After transcription, the 3′-end is oligo-uridylylated by a terminal uridylyltransferase, TUT1 (TUTase6)910, one of the members of the non-canonical nucleotidyltransferases. TUT1 is composed of N-terminal Zn-finger, RRM, palm, fingers and KA-1 domains. The C-terminal region of TUT1 is a previously unidentified RNA-binding domain, and it was named the KA-1 domain. Thus, the present structural and biochemical studies have demonstrated that TUT1 acts as a U6 snRNA-specific terminal uridylyltransferase.

The crystal of TUT1 lacking the N-terminal Zn-finger, PRR and C-terminal region (TUT1_ΔC) was also obtained (form-IV). The crystal belongs to the space group P43212. The structure was modelled and refined to an R factor of 20.3% (Rfree of 24.2%) up to 3.2 Å resolution. In the form-IV TUT1_ΔC structure, the N-terminal domain adopts a typical RRM fold, with four anti-parallel β-sheets stacked onto two α-helices. A comparison of the structures of the N-terminal RRM of TUT1 and the U2AF65 RRM1 suggested that the conserved aromatic or hydrophobic resides (Phe59, Phe94 and Ile96) on the β-strands would be involved in single-stranded RNA binding. The linker region (residues 127–144), bridging the RRM and the fingers, was disordered and the electron density was not observed. Since the RRM does not interact with other domains in TUT1_ΔC in the crystal structure, the N-terminal RRM would be mobile in the substrate RNA-free form of TUT1. The N-terminal RRM is mobile relative to the catalytic core domains, and the C-terminal domain KA-1 domain rotates relative to the catalytic core domains.

>[4x]MGLRSVFVSGFPRDVDSAQLSEYFLAFGPVASVVMDKDKGVFAIVEMGDVGAREAVLSQSQHSLGGHRLRVRPREQKEFQSPASKSPKGAAPDSHQLAKALAEAADVGAQMIKLVGLRELSEAERQLRSLVVALMQEVFTEFFPGCVVHPFGSSINSFDVHGCDLDLFLDLGDLEEPQPVPKLPPASPLLEDREEGDLGKASELAETPKEEKAEGAAMLELVGSILRGCVPGVYRVQTVPSARRPVVKFAHRPSGLHGDVSLSNRLALHNSRFLSLASELDGRVRPLVYTLRAWAQGRGLSGSGPLLSNYALTLLVIYFLQTRDPPVLPTVSQLTQKAGEGEQVEVDGWDCSFPRDASRLEPSINVEPLSSLLAQFFSAVSSWDLRGSLLSLREGQALPVAGGLPSNLWEGLRLGPLNLQDPFDLSHNVAANVTSRVAGRLQNCCRAAANYARSLQYQRRSSRGRDWGLLPLLQPSSLEHHHHHH>IVGGYTCAANSIPYQVSLNSGSHFCGGSLINSQWVVSAAHCYKSRIQVRLGEHNIDVLEGNEQFINAAKIITHPNFNGNTLDNDIMLIKLSSPATLNSRVATVSLPRSCAAAGTECLISGWGNTKSSGSSYPSLLQCLKAPVLSDSSCKSSYPGQITGNMICVGFLEGGKDSCQGDSGGPVVCNGQLQGIVSWGYGCAQKNKPGVYTKVCNYVNWIQQTIAAN[2x];>KPDFCFLEEDPGICRGYITRYFYNNQTKQ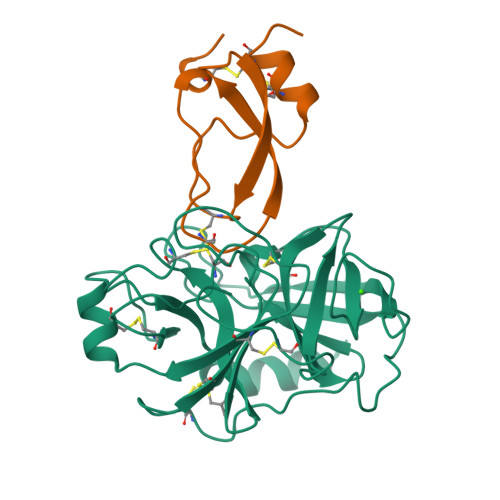CERFKYGGCLGNMNNFETLEECKNICEDG[2x]> MTPTQNVPEDRIQIGQLRSAYGLNGWLWVYSNTEPMSNMFDYLPWYIETKAGWQTVDVKRWKPHGKGLVVSLKGVSDRTGAESLVASNIWIAKSQLPKADVDEYYWSDLKGLTVLGLDDEEQEVNLGQIHELFETGANDVMVVRATPDSI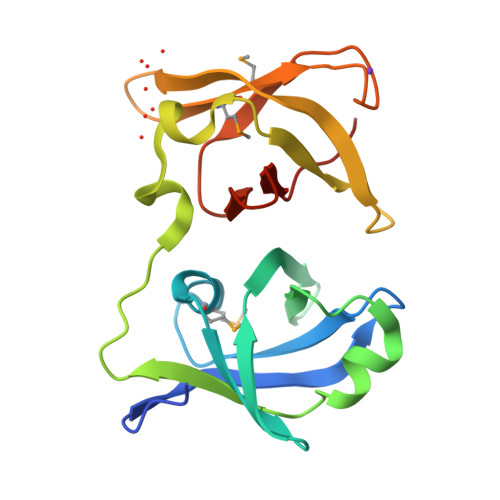DSEERMIPWHKDVVQRVDLEAGRIYVNWGVDY> SMAATAAEAVASGSGEPREEAGALGPAWDESQLRSYSFPTRPIPRLSQSDPRAEELIENEEPVVLTDTNLVYPALKWDLEYLQENIGNGDFSVYSASTHKFLYYDEKKMANFQNFKPRSNREEMKFHEFVEKLQDIQQRGGEERLYLQQTLNDTVGRKIVMDFLGFNWNWINKQQGKRGWGQLTSNLLLIGMEGNVTPAHYDEQQNFFAQIK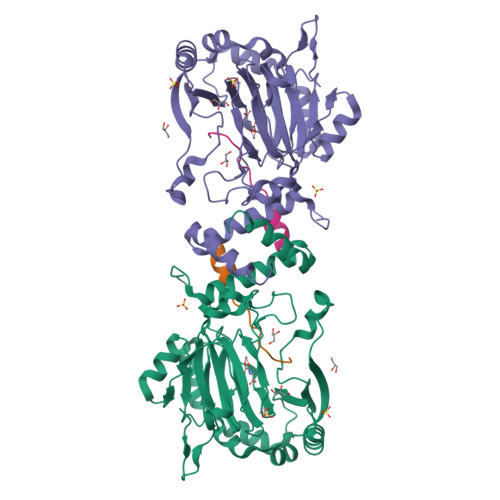GYKRCILFPPDQFECLYPYPVHHPCDRQSQVDFDNPDYERFPNFQNVVGYETVVGPGDVLYIPMYWWHHIESLLNGGITITVNFWYKGAPTPKRIEYPLKAHQKVAIMRNIEKMLGEALGNPQEVGPLLNTMIKGRYN;> GANYSIVDFLITAGANVNSPDSHG>[2x]SNAMLRRLFKKKYVCVRQYDLTDCGAACLSSIAQYYGLKMSLAKIREMTGTDTQGTNAYGLIHAAKQLGFSAKGVKASKEDLLKDFRLPAIANVIVDNRLAHFVVIYSIKNRIITVADPGKGIVRYSMDDFCSIWTGGLVLLEPGEAFQKGDYTQNMMVKFAGFLKPLKKTVLCIFLASLLYTALG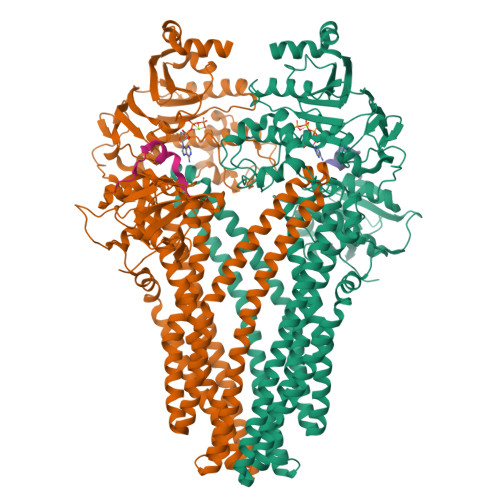IAGSFYIKFLFDDLIKFEKLNDLHIISAGFAVIFLLQIFLNYYRSILVTKLGMSIDKSIMMEYYSHVLKLPMNFFNSRKVGEIISRFMDASKIRQAISGATLTIMIDTIMAVIGGILLYIQNSSLFFISFIIILLYGIIVTVFNKPIQNANRQIMEDNAKLTSALVESVKGIETIKSFGAEEQTEKSTRDKIETVMKSSFKEGMLYINLSSLTGIVAGLGGIVILWAGAYNVIKGNMSGGQLLAFNALLAYFLTPVKNLIDLQPLIQTAVVASNRLGEILELATEKELREDSDDFVISLKGDIEFRNVDFRYGLRKPVLKNINLTIPKGKTVAIVGESGSGKTTLAKLLMNFYSPEKGDILINGHSIKNISLELIRKKIAFVSQDVFIFSGTVKENLCLGNENVDMDEIIKAAKMANAHDFIEKLPLKYDTFLNESGANLSEGQKQRLAIARALLKKPDILILDEATSNLDSITENHIKDAIYGLEDDVTVIIIAHRLSTIVNCDKIYLLKDGEIVESGSHTELIALKGCYFKMWKQTENTLAS;>SNAMSEAKKLNIGRELTDEELMEMTGGSTFSIQCQKDYTYKPSLPVVKYGVVIDEPEVVIKYGVGPIVGIKYGVEPIGPIQPMYGIKPVETLK[2x]>[2x]MHKVVIVGRPNVGKSSLFNRLLKKRSAVVADVPGVTRDLKEGVVETDRGRFLLVDTGGLWSGDKWEKKIQEKVDRALEDAEVVLFAVDGRAELTQADYEVAEYLRRKGKPVI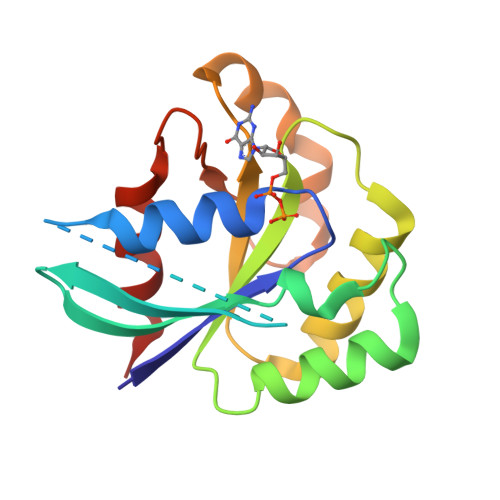LVATKVDDPKHELYLGPLYGLGFGDPIPTSSEHARGLEELLEAIWERLP>[2x]MKRMEANKIKLINEDNLRLDGRSFNELRPIKIQAGVLNRADGSAYIEWGGNKIMVGVYGPKEAYPKHSQDIDHAIVKARYNMAAFSVDERKRPGPDRRTMEISKVISEALSSSIMIEQFPRAEIDVYIEVLQADAGTRIAGLTAATVALADAGVPMRDMVVGCTAGKVDGHMVLDLSK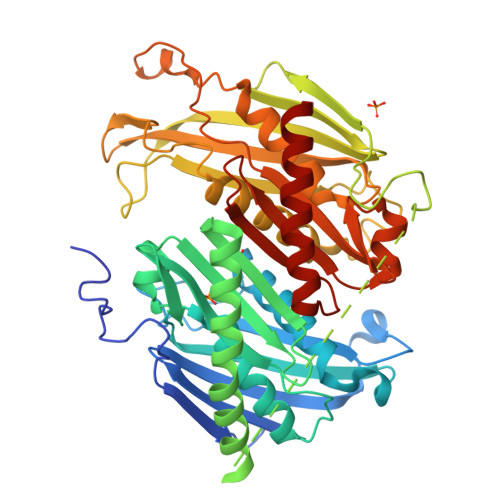EEDNYGEADIPIAIMPKTGDIVLMQMDGDVTEDELYQAMDMIFEATKRISQIQREALLNKYKIQDIGEGEMVKESAEILSEIRKNYILSTMKGGKRIDGRLPDEFRELTIIENYIPRANGSAYVALGNTRVVAGVKIEAGEPFPDTPDQGVLTTNVELLPIAFPSFEAGPPNDLAIEVSRVVDRGIRESKMISPEKLVIEQGKKVWIVFLDINVLDYDGNLIDASTIAAVAALRNAVVPASKEGGEDFKLPVSSTPISVTMVKIGDTLVCDPSLEEDQICGGRITVTTTEDGHIRAMQKGEIGAFTVEDVKKAVKMSLEVGKKLREKYFR>[4x]NISDTALTNELIHLLGHSRHDWMNKLQLIKGNLSLQ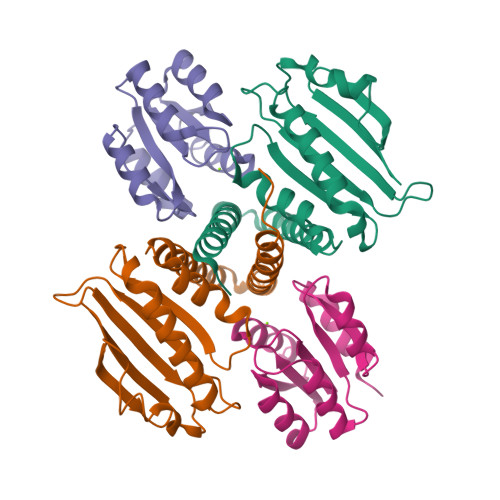KYDRVFEMIEEMVIDAKHESKLSNLKTPHLAFDFLTFNWKTHYMTLEYEVLGEIKDLSAYDQKLAKLMRKLFHLFDQAVSRESENHLTVSLQTDHPDRQLILYLDFHGAFADPSAFDDIRQNGYEDVDIMRFEITSHECLIEIGLD;>[4x]NEKILIVDDQSGIRILLNEVFNKEGYQTFQAANGLQALDIVTKERPDLVLLDMKIPGMDGIEILKRMKVIDENIRVIIMTAYGELDMIQESKELGALTHFAKPFDIDEIRDAVKKYLPL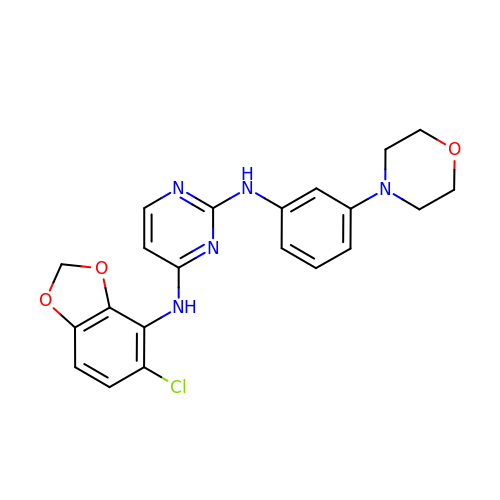N'-(5-CHLORO-1,3-BENZODIOXOL-4-YL)-N-(3-MORPHOLIN-4-YLPHENYL)PYRIMIDINE-2,4-DIAMINE | C21 H20 Cl N5 O3 | PNEWIQAEGKQNCE-UHFFFAOYSA-N>[2x]MRGSHHHHHHGSEARRSADYEPN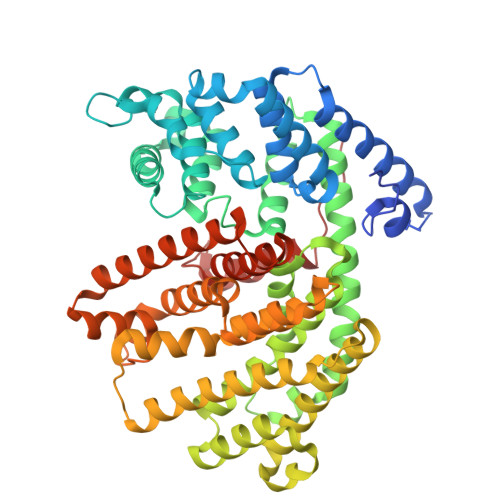SWDYDFLLSSDTDESIEVYKDKAKKLEAEVRREINNEKAEFLTLLELIDNVQRLGLGYRFESDIRRALDRFVSSGGFDGVTKTSLHATALSFRLLRQHGFEVSQEAFSGFKDQNGNFLENLKEDTKAILSLYEASFLALEGENILDEARVFAISHLKELSEEKIGKELAEQVNHALELPLHRRTQRLEAVWSIEAYRKKEDANQVLLELAILDYNMIQSVYQRDLRETSRWWRRVGLATKLHFARDRLIESFYWAVGVAFEPQYSDCRNSVAKMFSFVTIIDDIYDVYGTLDELELFTDAVERWDVNAINDLPDYMKLCFLALYNTINEIAYDNLKDKGENILPYLTKAWADLCNAFLQEAKWLYNKSTPTFDDYFGNAWKSSSGPLQLIFAYFAVVQNIKKEEIENLQKYHDIISRPSHIFRLCNDLASASAEIARGETANSVSCYMRTKGISEELATESVMNLIDETWKKMNKEKLGGSLFAKPFVETAINLARQSHCTYHNGDAHTSPDELTRKRVLSVITEPILPFER> QKPKTEIEMVVEQIIETQKQLNIEKLPSPWLPPLPPRLARPASVTAEANAFPIGLKDEPELQSQSDYFYQWLEDGNIGIFGSAGYGKSTTMMTLLLSFAGAYNPAQLHYYIFDFGNSALLPLRQLPHTADYFRLDDEKKIEKFIKF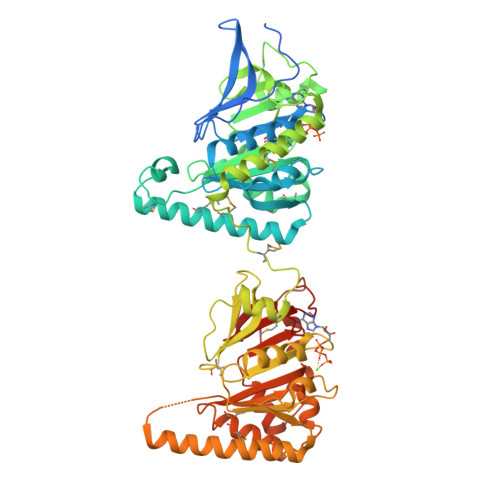MKEEMEQRKQRFMEKEVSTIKLYNALSEEKLPIIIVALDNFDVVKEEMPDFETQLIQYARDGQSLGIFFIMTATRVSGIRPPLMNNLKTKIVHYFIDSSEKFSLIGRTPYDVDPIPGRALIKKDNAALTQIYLPADGEDDIEVLENVKREMERLKEVYQHIPKPKPIPMLPPRLSMSVFTNTYVQHRASGFIPVGLDEQTVRPVAINMRTDPHCLIVGQSRKGKTNVVKVILESLLVQEPESIGLLDGIDRGLAGYANRDDITYIEAKERLAQWLNEADAVLQQREREYIQAVNENRATTLAWPPVVFVVDSLLRLQQETDSIMQGRIANMMKQYSHLGFHVFVAGNANEFVKGFDALTAELKQIRQAILVTKKSEQSLFALPFTRNEQEIEPGFGYFVVGGKDQKIQIPKVE> GTHLLFAQTGKIERLPLERNTMKKTEAKAFLHIPAKVIIGLAFDCVDKVVYWTDISEPSIGRASLHGGEPTTIIRQDLGSPEGIALDHLGRT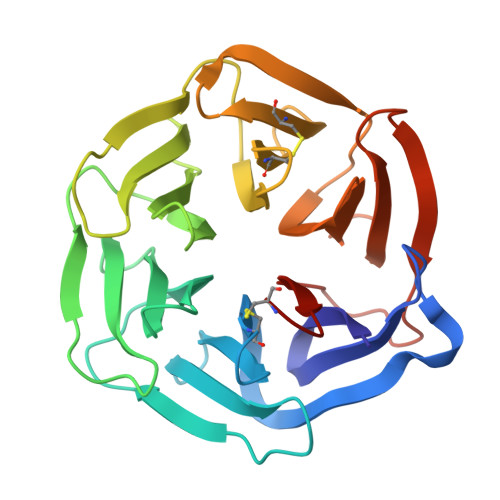IFWTDSQLDRIEVAKMDGTQRRVLFDTGLVNPRGIVTDPVRGNLYWTDWNRDNPKIETSHMDGTNRRILAQDNLGLPNGLTFDAFSSQLCWVDAGTHRAECLNPAQPGRRKVLEGLQYPFAVTSYGKNLYYTDWKTNSVIAMDLAISKEMDTFHPHKQTRLYGITIALSQCPQGH>[2x]GPGSTVNEQVQAWESRRPLIQDLARRLLTDDEVLAVTRHCSRYVHEGGVEDLVRPLL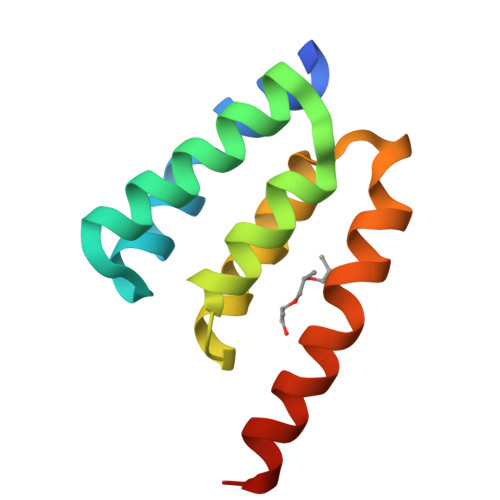AILDRPTKLLLLRDIRSVVAPTDLGRFDSMVMPVELEAFEALKSRAVG>MEALLEKAANPPAATVEAPPALFNFAAYLFRLNETRAGKTAYIDDTGSTTYGELEERARRFASALRTLGVHPEERILLVMLDTVALPVAFLGALYAGVVPVVANTLLTPADYVYMLTHSHARAVIASGALVQNVTQALESAEHDGCQLIVSQPRESEPRLAPLFEELIDAAAPAAKAAATGCDDIAFWLYSSGSTGKPKGTVHTHANLYWTAELYAKPILGIAENDVVFSAAKLFFAYGLGNGLTFPLSVGATAILMAERPTADAIFARLVEHRPTVFYGVPTLYANMLVSPNLPARADVAIRICTSAGEALPREIGERFTAHFGCEILDGIGSTEMLHIFL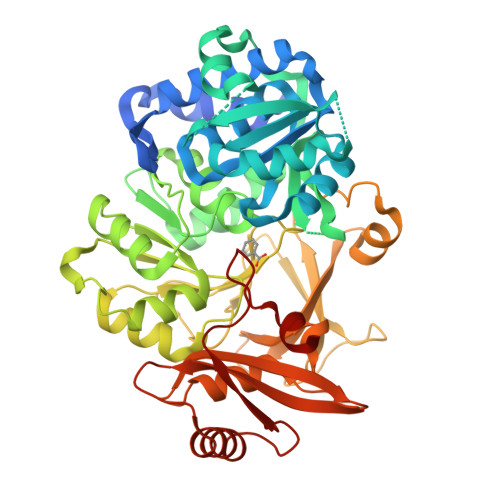SNRAGAVEYGTTGRPVPGYEIELRDEAGHAVPDGEVGDLYIKGPSAAVMYWNNREKSRATFLGEWIRSGDKYCRLPNGCYVYAGRSDDMLKVSGQYVSPVEVEMVLVQHDAVLEAAVVGVDHGGLVKTRAFVVLKREFAPSEILAEELKAFVKDRLAPHKYPRDIVFVDDLPKTATGKIQRFKLREQ[2x]>MHHHHHHENLYFQGRFDNKVVVITGAGNGMGEAAARRFSAEGAIVVLADWAKEAVDKVAASLPKGRAMAVHIDVSDHVAVEKMMNEVAEKLGRIDVLLNNAGVHVAGSVLETSIDDWRRIAGVDIDGVVFCSKFALPHLLKTKGCIVNTASVSGLGGDWGAAYYCAAKGAVVNLTRAMALDHGGDGVRINSVCPSLVKTNMTNGWPQEIRDKFNERIALGRAAEPEEVAAVMAFLASDDASFINGANIPVDGGATASDG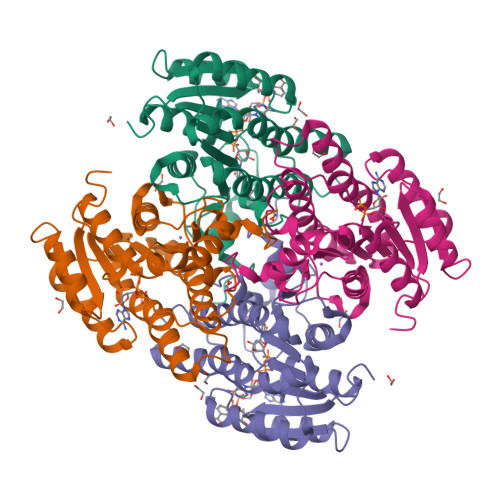APKIV[2x]> DRHHHHHHKLSVPSEDQPGDSYSHGQSCLGCVVLVSVIEQLAEVHNSSVQVAMERLCSYLPEKLFLKTACYFLVQTFGSDIIKLLDEAMKADVVCYALEFCKRGAVQPQCHLYPLPQEAWESALEKARQVLRRSSTMKYRRSGRNICSLPFLTKICQKIELSIKKAVPFKDVDSDKHSVFPTLRGYHWRGRDCNDSDKTVYPGRRPDNWDIHQDSNCNGIWGIDPKDGIPYEKKFCEGSQPRGIILLGDAAGAHFHIPPEWLTASQMSVNSFLNLPSALTDELNWPQLSGVTGFLDSTSGIEEKSIYHRLRKRNHCNHRDYQSISK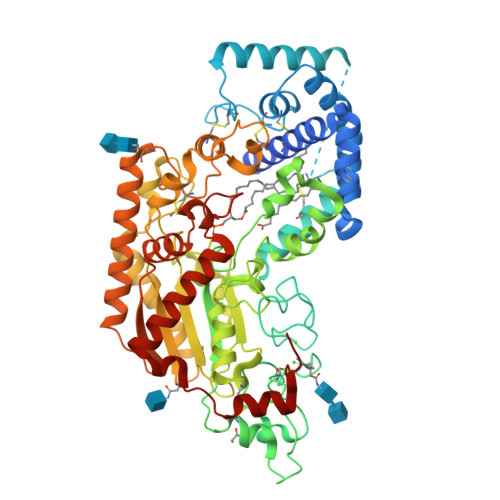NGASSRNLKNFIESLSRNQASDHPAIVLYAMIGNDVCNSKADTVPEMTTPEQMYANVMQTLTHLNSHLPNGSHVILYGLPDGTFLWDSLHNRYHPLGQLNKDVTYAQFFSFLRCLQLNPCNGWMSSNKTLRTLTSERAEQLSNTLKKIATTETFANFDLFYVDFAFHEIIEDWQKRGGQPWQLIEPVDGFHPNEVASLLQANRVWEKIQLQWPHVLGKENPFNSQIEEVFGDQGGH> MEPQDPVKREGRLTPVIVLATLIAAFGSSFQYGYNVAAINSPSEFMKDFYAYTYYDRVGEYMNEFYLTLLWSVTVSMFPFGGFLGSLMVGPLVNNLGRKGTLLFNNIFSIVPALLMGFSELAKSFEMIIVARVLVGICAGLSSNVVPMYLGELAPKNWRGALGVVPQLFITIGILVAQIFGLRSLLANEEGWPILLGLTGIPAVLQLLFLPFFPESPRYLLIQKKDEAAAKSALRRLRGWH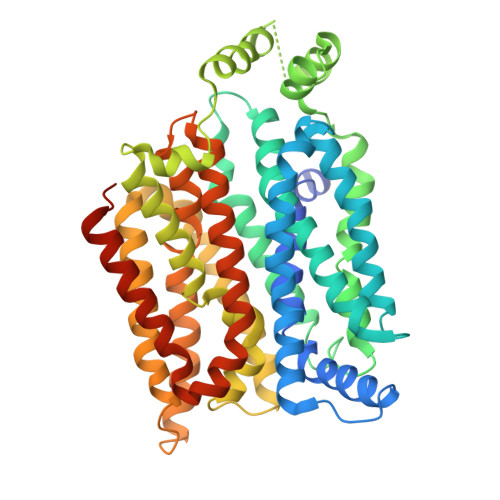DVDAEIEEILEEDRAEKAVGFISVLKLFKMRSLRWQVISIIVLMAGQQLSGVNAIYYYADQIYLSAGVNEDDVQYVTAGTGAVNVLITVCAIFVVELMGRRFLLLLGFSVCFTACCVLTGALALQDVISWMPYVSIACVISYVIGHALGPSPIPALLVTEIFLQSSRPAAYMVAGTVHWLSNFTVGLVFPFIQVGLGAYSFVIFAVICLLTTVYIFLIIPETKSKTFIEINRENLYFQ>[2x]MAAHRPVEWVQAVVSRFDEQLPIKTGQQNTHTKVSTEHNKECLINISKYKFSLVISGLTTILKNVNNMRIFGEAAEKNLYLSQLIILDTLEKCLAGQPKDTMRLDETMLVKQLLPEICHFLHTCREGNQHAAELRNSASGVLFSLSCNNFNAVFSRISTRLQELTVCSEDNVDVHDIELLQYINVDCAKLKRLLKETAFKFKALKKVAQLAVINSLEKAFWNWVENYPDEFTKLYQIPQTDMAECAEKLFDLVDGFAESTKRKAAVWPLQIILLILCPEIIQDISKDVVDENNMNKKLFLDSLRKALAGHGGSRQLTESAAIACVKLCKASTYINWEDNSVIFLLVQSMVVDLKNLLFNPSKPFSRGSQPADVDLMIDCLVSCFRISPHNNQHFKICLAQNSPSTFHYVLVNSLHRIITNSALDWWPKIDAVYCHSVELRNMFGETLHKAVQGCGAHPAIRMAPSLTFKEKVTSLKFKEKPTDLETRSYKYLLLSMVKLIHADPKLLLCNPRKQGPETQGSTAELITGLVQLVPQSHMPEIAQEAMEALLVLHQLDSIDLWNPDAPVETFWEISSQMLFYICKKLTSHQMLSSTEILKWLREILICRNKFLLKNKQADRSSCHFLLFYGVGCDIPSSGNTSQMSMDHEELLRTPGASLRKGKGNSSMDSAAGCSGTPPICRQAQTKLEVALYMFLWNPDTEAVLVAMSCFRHLCEEADIRCGVDEVSVHNLLPNYNTFMEFASVSNMMSTGRAALQKRVMALLRRIEHPTAGNTEAWEDTHAKWEQATKLILNYPKAKMEDGQAAESLHKTIVKRRMSHVSGGGSIDLSDTDSLQEWINMTGFLCALGGVCLQQRSNSGLATYSPPMGPVSERKGSMISVMSSEGNADTPVSKFMDRLLSLMVCNHEKVGLQIRTNVKDLVGLELSPALYPMLFNKLKNTISKFFDSQGQVLLTDTNTQFVEQTIAIMKNLLDNHTEGSSEHLGQASIETMMLNLVRYVRVLGNMVHAIQIKTKLCQLVEVMMARRDDLSFCQEMKFRNKMVEYLTDWVMGTSNQAADDDVKCLTRDLDQASMEAVVSLLAGLPLQPEEGDGVELMEAKSQLFLKYFTLFMNLLNDCSEVEDESAQTGGRKRGMSRRLASLRHCTVLAMSNLLNANVDSGLMHSIGLGYHKDLQTRATFMEVLTKILQQGTEFDTLAETVLADRFERLVELVTMMGDQGELPIAMALANVVPCSQWDELARVLVTLFDSRHLLYQLLWNMFSKEVELADSMQTLFRGNSLASKIMTFCFKVYGATYLQKLLDPLLRIVITSSDWQHVSFEVDPTRLEPSESLEENQRNLLQMTEKFFHAIISSSSEFPPQLRSVCHCLYQATCHSLLNKATVKEKKENKKSVVSQRFPQNSIGAVGSAMFLRFINPAIVSPYEAGILDKKPPPRIERGLKLMSKILQSIANHVLFTKEEHMRPFNDFVKSNFDAARRFFLDIASDCPTSDAVNHSLSFISDGNVLALHRLLWNNQEKIGQYLSSNRDHKAVGRRPFDKMATLLAYLGPPEHKPVADTHWSSLNLTSSKFEEFMTRHQVHEKEEFKALKTLSIFYQAGTSKAGNPIFYYVARRFKTGQINGDLLIYHVLLTLKPYYAKPYEIVVDLTHTGPSNRFKTDFLSKWFVVFPGFAYDNVSAVYIYNCNSWVREYTKYHERLLTGLKGSKRLVFIDCPGKLAEHIEHEQQKLPAATLALEEDLKVFHNALKLAHKDTKVSIKVGSTAVQVTSAERTKVLGQSVFLNDIYYASEIEEICLVDENQFTLTIANQGTPLTFMHQECEAIVQSIIHIRTRWELSQPDSIPQHTKIRPKDVPGTLLNIALLNLGSSDPSLRSAAYNLLCALTCTFNLKIEGQLLETSGLCIPANNTLFIVSISKTLAANEPHLTLEFLEECISGFSKSSIELKHLCLEYMTPWLSNLVRFCKHNDDAKRQRVTAILDKLITMTINEKQMYPSIQAKIWGSLGQITDLLDVVLDSFIKTSATGGLGSIKAEVMADTAVALASGNVKLVSSKVIGRMCKIIDKTCLSPTPTLEQHLMWDDIAILARYMLMLSFNNSLDVAAHLPYLFHVVTFLVATGPLSLRASTHGLVINIIHSLCTCSQLHFSEETKQVLRLSLTEFSLPKFYLLFGISKVKSAAVIAFRSSYRDRSFSPGSYERETFALTSLETVTEALLEIMEACMRDIPTCKWLDQWTELAQRFAFQYNPSLQPRALVVFGCISKRVSHGQIKQIIRILSKALESCLKGPDTYNSQVLIEATVIALTKLQPLLNKDSPLHKALFWVAVAVLQLDEVNLYSAGTALLEQNLHTLDSLRIFNDKSPEEVFMAIRNPLEWHCKQMDHFVGLNFNSNFNFALVGHLLKGYRHPSPAIVARTVRILHTLLTLVNKHRNCDKFEVNTQSVAYLAALLTVSEEVRSRCSLKHRKSLLLTDISMENVPMDTYPIHHGDPSYRTLKETQPWSSPKGSEGYLAATYPTVGQTSPRARKSMSLDMGQPSQANTKKLLGTRKSFDHLISDTKAPKRQEMESGITTPPKMRRVAETDYEMETQRISSSQQHPHLRKVSVSESNVLLDEEVLTDPKIQALLLTVLATLVKYTTDEFDQRILYEYLAEASVVFPKVFPVVHNLLDSKINTLLSLCQDPNLLNPIHGIVQSVVYHEESPPQYQTSYLQSFGFNGLWRFAGPFSKQTQIPDYAELIVKFLDALIDTYLPGIDEETSEESLLTPTSPYPPALQSQLSITANLNLSNSMTSLATSQHSPGIDKENVELSPTTGHCNSGRTRHGSASQVQKQRSAGSFKRNSIKKIV

The autosomal dominant monogenetic disease neurofibromatosis type 1 (NF1) affects approximately one in 3,000 individuals and is caused by mutations in the NF1 tumour suppressor gene, leading to dysfunction in the protein neurofibromin (Nf1). As a GTPase-activating protein (GAP), its primary function is suppression of the Ras signalling cascade by accelerating the GTP hydrolysis rate of Ras, which returns Ras to its inactive GDP bound form. The ubiquitous Nf1 isoform-2 splice variant Nf1-23a (2839aa) is, together with Nf1 isoform 1, which lacks the 23a insertion (2818aa), one of the two biologically relevant alternative Nf1 isoforms. Our high-resolution single particle cryo-electron microscopy (EM) structures reveal the domain organization and structural details of the full-length Nf1-23a isoform 2 dimer.

Three major dimer interfaces between the protomers exist in both states. The N-terminal HEAT helices contact the terminal C-HEAT helices at the other protomer, each contact burying about 950 Å2 of surface area. The resulting dimer is connected in the centre, forming a core that buries almost 3,000 Å2 of surface area. The Nf1 HEAT/ARM dimer framework is rigid in its core, providing a stable platform for the GRD-Sec14-PH domain rearrangement while retaining high mobility at the peripheral tips of the two lobes. The disordered, S-rich region branching out from C-HEAT helix α103 and returning into the core at C-HEAT helix α104 could not be traced. Flexibility and solvent access are consistent with the reported target for phosphorylation.> MSNKERFLTLYHQIKSDANGYFSPEGIPYHSIETLICEAPDYGHMTTSEAYSYWLWLEVLYGHYTRDWSKLEAAWDNMEKYIIPVNEDGNDEQPHMSAYNPSSPATYASEKPYPDQYPSQLSGARPAGQDPIDGELKSTYGTNETYLMHWLLDVDNWYKYGNLLNPSHKAAYVNTFQRGQQESVWEAIPHPSQDDKSFGKPNEGFMSLFTKENQVPAAQWRYTNATDADARAIQAIYWAKELGYNNSTYLDKAKKMGDFLRYGMYDKYFQTIGSGKQGNPYPGNGKGACHYLMAWYTSWGGGLGDYANWSWRIGASHCHQGYQNPVAAYALSSDKGGLKPSSATGASDWEKTLKRQLEFYVWLQSKEGAIAGGATNSWNGDYSAYPAGRSTFYDMAYEDAPVYHDPPSNNWFGMQAWPMERVA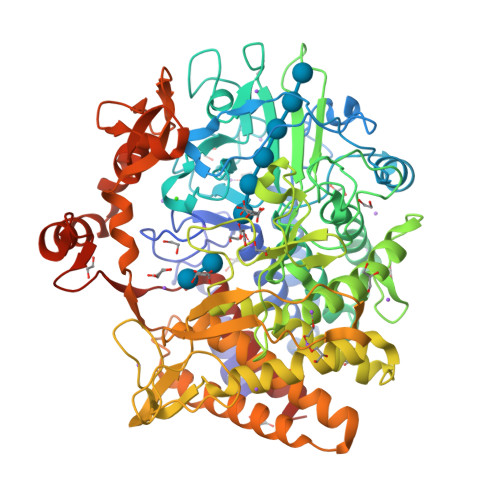ELYYIFVKDGDKTSENVQMAKSCITKWVNYALDYIFIGSRPVSDEEGYFLDDQGRRILGGTNATVATTSAPGEFWLPGNIAWSGQPDTWNGFQSATGNPNLTAVTKDPTQDTGVLGSLVKAFTFFAAATKLETGNYTALGVRAKDAAAQLLEVAWNYNDGVGIVTEEEREDYDRFFKKEVYFPNGWNGTFGQGNQIPGSSTIPSDPQRGGNGVYTSFADLRPNIKQDPAWSSLESKYQSSFNEATGKWENGAPVFTYHRFWSQVDMATAYAEYHRLINLEHHHHHH Condensin protein complexes coordinate the formation of mitotic chromosomes and thereby ensure the successful segregation of replicated genomes. Here, we identify a direct DNA-binding site in the eukaryotic condensin complex, which is formed by its Ycg1Cnd3 HEAT-repeat and Brn1Cnd2 kleisin subunits. A peptide loop of the kleisin subunit encircles the bound DNA and, like a safety belt, prevents its dissociation. Firm closure of the kleisin loop around DNA is essential for the association of condensin complexes with chromosomes and their DNA-stimulated ATPase activity.

To gain detailed insight into the nature of the DNA binding site, we solved crystal structures of the Ycg1–Brn1 subcomplex of Saccharomyces cerevisiae (Sc) and of the homologous Cnd3–Cnd2 subcomplex of Schizosaccharomyces pombe (Sp) to 2.8 Å and 2.6 Å resolution, respectively. Both structures are strikingly similar and reveal a harp-shaped conformation of the HEAT-repeat subunit, with the kleisin subunit winding along the concave surface of the HEAT-repeat solenoid. The peculiar curvature of Ycg1 and Cnd3 has its cause in three discontinuities in the directionality of the solenoid formed by the 19 HEAT-repeat motifs. The Brn1 kleisin subunit makes extended contacts with the inner surface of the Ycg1 harp, burying a total surface area of 3,754 Å2. Through multiple hydrophobic, electrostatic, and hydrogen bond interactions with the HEAT-repeat subunit, Brn1 forms a rigid “bridge” between the two Ycg1 lobes. One of the two molecules in the asymmetric unit of the Ycg1–Brn1 and Cnd3–Cnd2 crystals shows additional electron density for a segment that corresponds to a long helix (α1) in the N-terminal region of the kleisin subunit. This helix and the succeeding well-ordered turn stack onto HEAT motifs 16 and 17 and onto the α4 segment of the kleisin via several highly conserved aromatic residues in a manner that resembles a “latch” that has been inserted into a “buckle”. Through the interaction of latch and buckle regions, the kleisin subunit adopts a loop configuration. The absence of density for the latch segment in half of the complexes suggests that the α2 to α4 segments of the kleisin subunit are sufficient for complex formation with the HEAT-repeat subunit. Mapping of the electrostatic surface potential onto the Sc Ycg1–Brn1 structure revealed that the wide groove between the two shoulders of the Ycg1 harp and the Brn1 bridge displays a high degree of positive surface charge.

>[2x]MGIDINTKIFNSVAEVFQKAQGSYAGHRKHIAVLKKIQSKAVEQGYEDAFNFWFDKLVTKILPLKKNEIIGDRIVKLVAAFIASLERELILAKKQNYKLTNDEEGIFSRFVDQFIRHVLRGVESPDKNVRFRVLQLLAVIMDNIGEIDESLFNLLILSLNKRIYDREPTVRIQAVFCLTKFQDEEQTEHLTELSDNEENFEATRTLVASIQNDPSAEVRRAAMLNLINDNNTRPYILERARDVNIVNRRLVYSRILKSMGRKCFDDIEPHIFDQLIEWGLEDRELSVRNACKRLIAHDWLNALDGDLIELLEKLDVSRSSVCVKAIEALFQSRPDILSKIKFPESIWKDFTVEIAFLFRAIYLYCLDNNITEMLEENFPEASKLSEHLNHYILLRYHHNDISNDSQSHFDYNTLEFIIEQLSIAAERYDYSDEVGRRSMLTVVRNMLALTTLSEPLIKIGIRVMKSLSINEKDFVTMAIEIINDIRDDDIEKQESESDIINNLPPEKEASSATIVLCLTRSSYMLELVNTPLTENILIASLMDTLITPAVRNTAPNIRELGVKNLGLCCLLDVKLAIDNMYILGMCVSKGNASLKYIALQVIVDIFSVHGNTVVDGEGKVDSISLHKIFYKVLKNNGLPECQVIAAEGLCKLFLADVFTDDDLFETLVLSYFSPINSSNEALVQAFAFCIPVYCFSHPAHQQRMSRTAADILLRLCVLWDDLQSSVIPEVDREAMLKPNIIFQQLLFWTDPRNLVNQTGSTKKDTVQLTFLIDVLKIYAQIEKKEIKKMIITNINAIFLSSEQDYSTLKELLEYSDDIAENDNLDNVSKNALDKLRNNLNSLIEEINERSETQTKDENNTANDQYSSILGN;>GPLGHMSIFEKDLMAYFDENLNRNWRGREHWKVRNFKKANLVNKESDLLEETRTTIGDTTDKNTTDDKSMDTKKKHKQKKVLEIDFFKTDDSFEDKVFASKGRTKIDMPIKNRKNDTHYLLPDDFHFSTDRITRLFIKPGQKMSLFSHRKHT[2x]> MAAA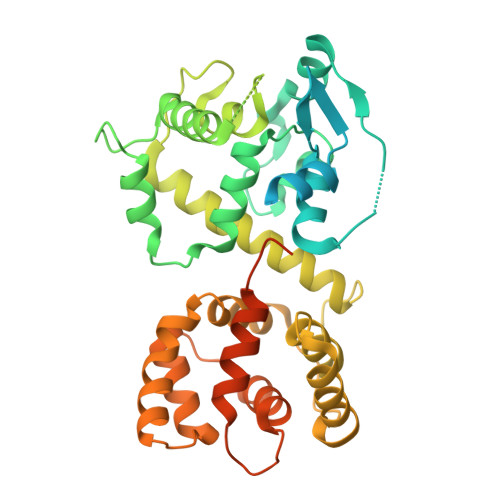AGSCARVAAWGGKLRRGLAVSRQAVRSPGPLAAAVAGAALAGAGAAWHHSRVSVAARDGSFTVSAQKNVEHGIIYIGKPSLRKQRFMQFSSLEHEGEYYMTPRDFLFSVMFEQMERKTSVKKLTKKDIEDTLSGIQTAGCGSTFFRDLGDKGLISYTEYLFLLTILTKPHSGFHVAFKMLDTDGNEMIEKREFFKLQKIISKQDDLMTVKTNETGYQEAIVKEPEINTTLQMRFFGKRGQRKLHYKEFRRFMENLQTEIQEMEFLQFSKGLSFMRKEDFAEWLLFFTNTENKDIYWKNVREKLSAGESISLDEFKSFCHFTTHLEDFAIAMQMFSLAHRPVRLAEFKRAVKVATGQELSNNILDTVFKIFDLDGDECLSHEEFLGVLKNRMHRGLWVPQHQSIQEYWKCVKKESIKGVKEVWKQAGKGLF>MRCIGISNRDFVEGVSGGSWVDIVLEHGSCVTTMAKNKPTLDFELIKTEAKQPATLRKYCIEAKLTNTTTDSRCPTQGEPTLNEEQDKRFVCKHSMVDRGWGNGCGLFGKGGIVTCAMFTCKKNMEGKIVQPENLEYTVVITPHSGEEHAVGNDTGKHGKEVKITPQSSITEAELTGYGTVTMECSPRTGLDFNEMVLLQMKDKAWLVHRQWFLDLPLPWLPGADTQGSNWIQKETLVTFKNP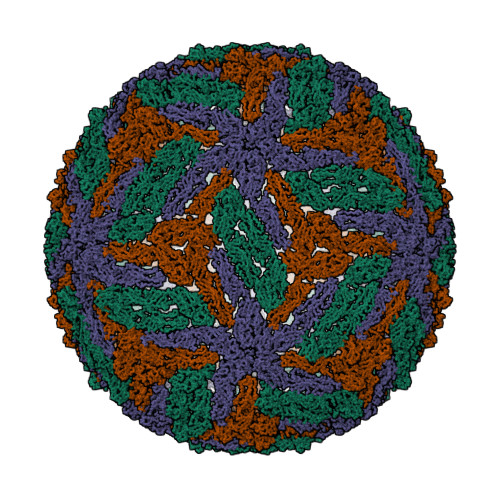HAKKQDVVVLGSQEGAMHTALTGATEIQMSSGNLLFTGHLKCRLRMDKLQLKGMSYSMCTGKFKVVKEIAETQHGTIVIRVQYEGDGSPCKIPFEIMDLEKRHVLGRLITVNPIVTEKDSPVNIEAEPPFGDSYIIIGVEPGQLKLDWFKKG[3x]>GGDPHMMFGKKKNNGGSSTARYSAGNKYNTLSNNYALSAQQLLNASKIDDIDSMMGFERYVPPQYNGRFDAKDIDQIPGRVGWLTNMHATLVSQETLSSGSNGGGNSNDGERVTTNQGISGVDFYFLDEEGGSFKSTVVYDPYFFIACNDESRVNDVEELVKKYLESCLKSLQIIRKEDLTMDNHLLGLQKTLIKLSFVNSNQLFEARKLLRPILQDNANNNVQRNIYNVAANGSEKVDAKHLIEDIREYDVPYHVRVSIDKDIRVGKWYKVTQQGFIEDTRKIAFADPVVMAFDIETTKPPLKFRDSAVDQIMMISYMIDGEGFLITNREIISEDIEDFEYTPKPEYPGFFTIFNENDEVALLQRFFEHIRDVRPTVISTFNGDFFDWPFIHNRSKIHGLDMFDEIGFAPDAEGEYKSSYCSHMDCFRWVKRDSYLPQGSQGLKAVTQSKLGYNPIELDPELMTPYAFEKPQHLSEYSVSDAVATYYLYMKYVHPFIFSLCTIIPLNPDETLRKGTGTLCEMLLMVQAYQHNILLPNKHTDPIERFYDGHLLESETYVGGHVESLEAGVFRSDLKNEFKIDPSAIDELLQELPEALKFSVEVENKSSVDKVTNFEEIKNQITQKLLELKENNIRNELPLIYHVDVASMYPNIMTTNRLQPDSIKAERDCASCDFNRPGKTCARKLKWAWRGEFFPSKMDEYNMIKRALQNETFPNKNKFSKKKVLTFDELSYADQVIHIKKRLTEYSRKVYHRVKVSEIVEREAIVCQRENPFYVDTVKSFRDRRYEFKGLAKTWKGNLSKIDPSDKHARDEAKKMIVLYDSLQLAHKVILNSFYGYVMRKGSRWYSMEMAGITCLTGATIIQMARALVERVGRPLELDTDGIWCILPKSFPETYFFTLENGKKLYLSYPCSMLNYRVHQKFTNHQYQELKDPLNYIYETHSENTIFFEVDGPYKAMILPSSKEEGKGIKKRYAVFNEDGSLAELKGFELKRRGELQLIKNFQSDIFKVFLEGDTLEGCYSAVASVCNRWLDVLDSHGLMLEDEDLVSLICENRSMSKTLKEYEGQKSTSITTARRLGDFLGEDMVKDKGLQCKYIISSKPFNAPVTERAIPVAIFSADIPIKRSFLRRWTLDPSLEDLDIRTIIDWGYYRERLGSAIQKIITIPAALQGVSNPVPRVEHPDWLKRKIA[2x]

At the eukaryotic replication fork, the family B replicative DNA polymerases epsilon (Pol ε) and delta (Pol δ) synthesize the leading and lagging strand, respectively. The exonuclease domains of family B polymerases have several highly-conserved motifs (named Exo-motifs), which include the catalytic residues (D290, E292, D383 and D477 in yeast Pol ε). The catalytic residues serve as ligands for two metal ions, and substituting both D290 and E292 with alanine abolishes the proofreading function of the polymerase, which in turn increases the in vitro mutation rate by ~100-fold. At present, many structures of family B DNA polymerases with proofreading capacity have been determined, and their overall structures are well conserved, consisting of a thumb, palm, fingers and the exonuclease domain.

Here we report the crystal structure of the catalytic core of S. cerevisiae Pol ε with a P301R substitution, orthologous to P286R in human Pol ε. The Pol2CORE-P301R was stable during the purification, gave a similar yield as the wild-type Pol2CORE, and crystallized readily in the presence of DNA and an incoming nucleotide. There were no rearrangements of the N-terminal, exonuclease, finger, palm, thumb or P-domains, nor were there any alterations in the interactions with DNA and the incoming nucleotide in the ternary complex of Pol2CORE-P301R. All considered, this suggests that the capacity of Pol2CORE-P301R to synthesize DNA should not be compromised. The overall crystal structure of the exonuclease domain of Pol2CORE-P301R is very similar to the wild-type structure. The P301R substitution is located in a loop, called the Exo-loop, but does not affect the overall conformation of the Exo-loop. In the Pol2CORE-P301R structure, the R301 points toward the catalytic site, forming an ion pair with E292. The R301-E292 ion pair interaction is buttressed by a water molecule that is stabilized by the backbone amide group of T293. In contrast to the wild-type, the P301R structure harbors only a Ca2+ ion in the A-site, coordinated by water molecules and three catalytic residues D290, E292 and D477. Interestingly, we observe a steric clash between the terminal residue of the ssDNA and R301, suggesting that R301 will interfere with the binding of ssDNA to the exonuclease site.> MGEVTAEEVEKFLDSNVSFAKQYYNLRYRAKVISDLLGPREAAVDFSNYHALNSVEESEIIFDLLRDFQDNLQAEKCVFNVMKKLCFLLQADRMSLFMYRARNGIAELATRLFNVHKDAVLEECLVAPDSEIVFPLDMGVVGHVALSKKIVNVPNTEEDEHFCDFVDTLTEYQTKNILASPIMNGKDVVAIIMVVNKVDGPHFTENDEEILLKYLNFANLIMKVFHLSYLHNCETRRGQILLWSGSKVFEELTDIERQFHKALYTVRAFLNCDRYSVGLLDMTKQKEFFDVWPVLMGEAPPYAGPRTPDGREINFYKVIDYILHGKEDIKVIPNPPPDHWALVSGLPTYVAQNGLICNIMNAPSEDFFAFQKEPLDESGWMIKNVLSMPIVNKKEEIVGVATFYNRKDGKPFDEMDETLMESLTQFLGWSVLNPDTYELMNKLENRKDIFQDMVKYHVKCDNEEIQTILKTREVYGKEPWECEEEELAEILQGELPDADKYEINKFHFSDLPLTELELVKCGIQMYYELKVVDKFHIPQEALVRFMYSLSKGYRRITYHNWRHGFNVGQTMFSLLVTGKLKRYFTDLEALAMVTAAFCHDIDHRGTNNLYQMKSQNPLAKLHGSSILERHHLEFGKTLLRDESLNIFQNLNRRQHEHAIHMMDIAIIATDLALYFKKRTMFQKIVDQSKTYETQQEWTQYMMLDQTRKEIVMAMMMTACDLSAITKPWEVQSKVALLVAAEFWEQGDLERTVLQQNPIPMMDRNKADELPKLQVGFIDFVCTFVYKEFSRFHEEITPMLDGITNNRKEWKALADEYETKMKGLEEEKQKQQAANQAAAGSQHGGKQPGGGPASKSCCVQ;> MSLSEGQVHRFLDQNPGFADQYFGRKLSPEDVANACEDGCPEGCTSFRELCQVEESAALFELVQDMQENVNMERVVFKILRRLCSILHADRCSLFMYRQRNGVAELATRLFSVQPDSVLEDCLVPPDSEIVFPLDIGVVGHVAQTKKMVNVQDVMECPHFSSFADELTDYVTRNILATPIMNGKDVVAVIMAVNKLDGPCFTSEDEDVFLKYLNFGTLNLKIYHLSYLHNCETRRGQVLLWSANKVFEELTDIERQFHKAFYTVRAYLNCDRYSVGLLDMTKEKEFFDVWPVLMGEAQAYSGPRTPDGREILFYKVIDYILHGKEDIKVIPSPPADHWALASGLPTYVAESGFICNIMNAPADEMFNFQEGPLDDSGWIVKNVLSMPIVNKKEEIVGVATFYNRKDGKPFDEQDEVLMESLTQFLGWSVLNTDTYDKMNKLENRKDIAQDMVLYHVRCDREEIQLILPTRERLGKEPADCEEDELGKILKEVLPGPAKFDIYEFHFSDLECTELELVKCGIQMYYELGVVRKFQIPQEVLVRFLFSVSKGYRRITYHNWRHGFNVAQTMFTLLMTGKLKSYYTDLEAFAMVTAGLCHDIDHRGTNNLYQMKSQNPLAKLHGSSILERHHLEFGKFLLSEETLNIYQNLNRRQHEHVIHLMDIAIIATDLALYFKKRTMFQKIVDESKNYEDRKSWVEYLSLETTRKEIVMAMMMTACDLSAITKPWEVQSKVALLVAAEFWEQGDLERTVLDQQPIPMMDRNKAAELPKLQVGFIDFVCTFVYKEFSRFHEEILPMFDRLQNNRKEWKALADEYEAKVKALEEDQKKETTAKKVGTEICNGGPAPRSSTCRIL;>MNLEPPKAEIRSATRVMGGPVTPRKGPPKFKQRQTRQFKSKPPKKGVQGFGDDIPGMEGLGTDITVICPWEAFNHLELHELAQYGII[2x]

Phototransduction in retinal rods occurs when the G protein–coupled photoreceptor rhodopsin triggers the activation of phosphodiesterase 6 (PDE6) by GTP-bound alpha subunits of the G protein transducin (GαT). PDE6 consists of two highly similar but not identical subunits (PDE6α and PDE6β, Mr ∼100 kDa), each containing a catalytic site and two domains (GAFa and GAFb) that mediate a negative allosteric regulation by cGMP, together with two smaller (identical) subunits (PDE6γ, Mr ∼10 kDa) that are the binding sites for GTP-bound GαT (GαT·GTP). PDE6 is a 3′,5′-cyclic nucleotide phosphodiesterase and a member of a superfamily of enzymes that play critical roles in compartmentalizing cyclic nucleotide signaling and regulating many physiological processes. PDE6 is the most catalytically active PDE and is the only family member that has coevolved an autoinhibitory PDE6γ subunit, which enables G-protein–stimulated activation and completely prevents basal activity in the absence of GαT.

We then used cryo-EM to solve a high-resolution structure of PDE6 bound to udenafil. The resulting cryo-EM map was refined to 2.9 Å resolution and the initial atomic model was generated using ModelAngelo. The catalytic cores of the apo- and udenafil-bound PDE6 are remarkably similar, with an overall RMSD of 0.3 Å when aligned by the PDE6α catalytic site; however, there is minimal cryo-EM map density for the C termini of the PDE6γ subunits, which bind near the PDE6 active sites in apo-PDE6, as well as a weakened density for the glycine-rich region of PDE6γ. The cryo-EM map has local resolution peaks at 2.7 Å for the catalytic cores with strong density for udenafil bound at both active sites on PDE6α and PDE6β and for cGMP bound at their GAF A domains. Overall, the motions of the udenafil-bound PDE6 complex were similar to what we observe for the apoenzyme. Across all three components, the cryo-EM map density for PDE6γ is diminished while moving along the variability coordinate axis. This indicates that the binding of udenafil weakens the association of the PDE6γ C terminus with the catalytic sites, due to steric clashes, which would enhance the ability of activated GαT subunits to bind and reposition the PDE6γ subunits away from the PDE6 catalytic sites. Our high-resolution structures lack cryo-EM density for the PDE6γ C terminus near the PDE6 catalytic core, indicating that when large orthosteric inhibitors such as udenafil (516.7 g/mol) bind to PDE6, the PDE6γ C-terminus clashes with the ligand at the active site but remains bound to the PDE6α and PDE6β subunits through interactions with the dimerization domain and the GAF domains.>[2x]SGTVKYTDAQIQRLREYGNGTYEQKVFEDLASRDAAFSKEMSVASTDNEKKIKGMIANPSRHGLTQLMNDIADALVAEGFIEVRTPIFISKDALARMTITEDKPLFKQVFWIDEKRALRPMLAPNLYSVMRDLRDHTDGPVKIFEMGSCFRKESHSGMHLEEFTMLALGDMGPRGDATEVLKNYISVVMKAAGLPDYDLVQEESDVYKETIDVEINGQEVCSAAVGPHYLDAAHDVHEPC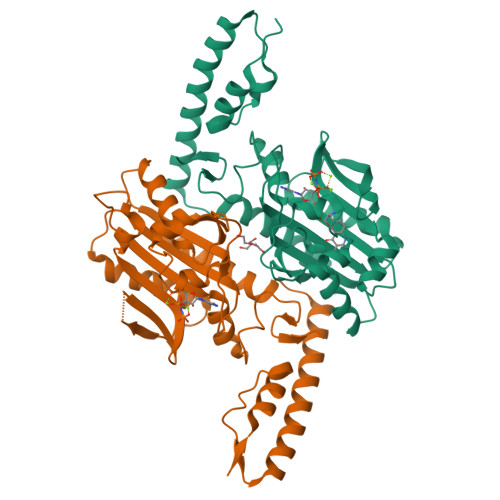SGAGFGLERLLTIREKYSTVKKGGASISYLNGAKIN>VTDLAGTTRLLRAQGVTAPAGFRAAGVAAGIKASGALDLALVFNEGPDYAAAGVFTRNQVKAAPVLWTQQVLTTGRLRAVILNSGGANACTGPAGFADTHATAEAVAAALSDWGTETGAIEVAVCSTGLIGDRLPMDKLLAGVAHVVHEMHGGLVGGDEAAHAIMTTDNVPKQVALHHHDNWTVGGMAKGAGMLAPSLA[2x];>[2x]TMLCVLTTDAAAEPAALERALRRAAAATFDRLDIDGSCSTNDTVLLLSSGASEIPPAQADLDEAVLRVCDDLCAQLQADAEGVTKRVTVTVTGAATEDDALVAARQIAR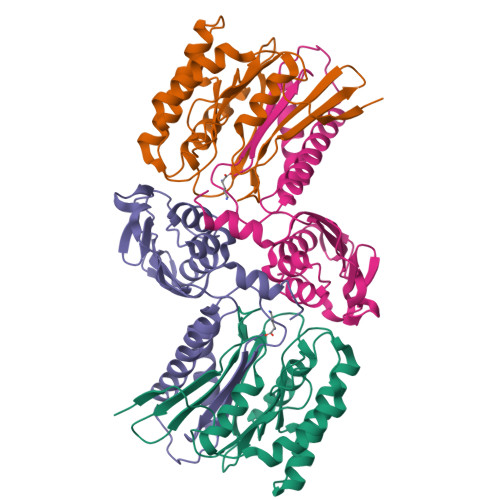DSLVKTALFGSDPNWGRVLAAVGMAPITLDPDRISVSFNGAAVCVHGVGAPGAREVDLSDADIDITVDLGVGDGQARIRTTDLSHAYVEENSAYSS> SETDDLKWTERLPECPVYRPTKEEFEDPLTYLQKIFPEASKYGICKIVSPLTATVPAGAVLMKEKSNFKFTTRVQPLRLAEWDSDDKVTFFMSGRTYTFRDYEKMANKVFARRYCSGGSLPDSFLEKEFWKEIACGKTETVEYACDVDGSAFSSAPGDPLGSSKWNLNKVSRLPKSTLRLLETSIPGVTEPMLYIGMLFSMFAWHVEDHYLYSINYQHCGASKTWYGIPGSAALKFEKVVKECVYNDDILSTNGEDGAFDVLLGKTTIFPPKTLLDHNVPVYKAVQKPGEFVVTFPRAYHAGFSHGFNCGEAVNFAMGDWFPFGAIASCRYAHLNRVPLLPHEELICKEAMLLNSSSKSENLDLTPTELSGQRSIKTAFVHLIRFLHLARWSLMKSGLCTGLVSNTYGTIVCSLCKRDCYLAFINCECYSHPVCLRHDVKKLDLPCGTTHTLYLRDNIEDMEAAAMKFEKEDGVSDLITTDEDLYKYPSS;> AARKSAPATGGV

Here we investigate the role of histone demethylases in plant flowering through the analysis of Arabidopsis JMJ13, which we show possesses H3K27me3 site-specific demethylase activity in vitro and in vivo. The recombinant expressed JMJ13 catalytic domain (JMJ13CD, residues 90–578) displayed unambiguous demethylation activity against H3K27me3 peptides, but not H3K4me3, H3K9me3, or H3K36me3 peptides, confirming that JMJ13 is an H3K27me3 site-specific histone demethylase. JMJ13 has a central catalytic domain flanked by flexible regions on both N- and C-termini. Our genetic studies suggest that JMJ13 acts as a flowering repressor, which modulates flowering time in a temperature- and photoperiod-dependent manner.

To investigate the substrate recognition and catalytic mechanism of JMJ13, we determined the crystal structure of JMJ13CD in complex with the α-KG analog N-oxalylglycine (NOG) and an H3K27me3 peptide, at 2.6 Å resolution. Overall the structure closely resembles the JMJ13-α-KG complex with a root-mean-square deviation (RMSD) of 0.49 Å. The peptide can be traced from H3A24 to H3A31. The peptide binds in a negatively charged cleft with the residues H3K27me3 to H3P30 located at the bottom of the cleft and the other flanking residues extending out from the cleft. The side chain of H3K27me3 inserts into a deep binding pocket within the active site cleft. An NOG molecule and a Ni2+ ion are deeply buried in the center of the active site. The interactions between JMJ13 and the H3K27me3 peptide are restricted to the region between H3R26 and H3P30. H3R26 forms salt bridge and hydrogen bonding interactions with Asp236 of JMJ13. H3P30 positions its side chain prolyl ring such that the plane of the propyl ring is parallel with and stacks on top of the phenyl ring of Phe179 of JMJ13, resulting in hydrophobic stacking and CH-π interactions. Compared with the JMJ13 peptide-free structure, the side chain of Phe179 undergoes a significant rotation to allow stacking with H3P30, indicative of a peptide binding-induced conformational change.2'-(4-HYDROXYPHENYL)-5-(4-METHYL-1-PIPERAZINYL)-2,5'-BI-BENZIMIDAZOLE | C25 H24 N6 O | 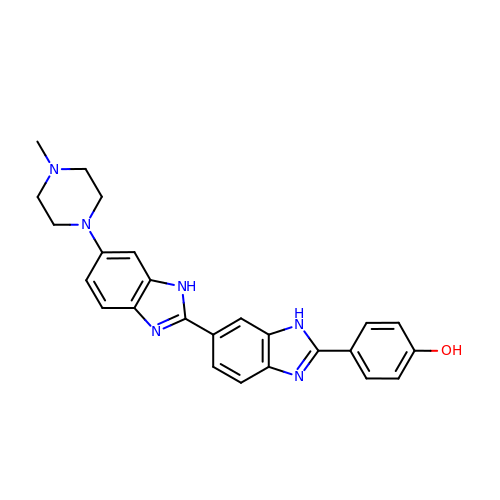INAAIJLSXJJHOZ-UHFFFAOYSA-N Cyclodipeptide synthases (CDPSs) use aminoacylated tRNA (aa-tRNA) substrates to form peptide bonds between two amino acids yielding a cyclic dipeptide product (CDP). ParaCDPS from Parabacteroides sp. 20_3 (GenBank: EFK64745.1) produces cyclo(His-Phe)8 whilst ParcuCDPS from Parcubacteria bacterium RAAC4_OD1_1 (GenBank: ETB63777.1) can synthesise both cyclo(His-Glu) and cyclo(His-Pro)9. ParcuCDPS belongs to the XYP sub-group of the CDPS family, characterised by the presence of 3 residues: X40 where X is a non-conserved residue, Y202, and P203 (numbering respective to AlbC). ParcuCDPS displays a Rossman-fold common throughout the CDPS family.

Inspired by HisRS and histidine recognition more generally, and by the only high resolution structure of a CDPS with a ligand bound, we systematically altered three unique residues in ParcuCDPS P1, which we hypothesised to be participating in crucial interactions with the polar side chain of histidine. We first designed Generation 1 containing seven P1 mutants (Y55F; Y55V; E174A; E174H; E174L; Y189F and Y189L), and these variants were cloned, expressed in E.coli, purified and used for activity assays. By mutating the P1 residues, the activity of the variants was vastly reduced with E174A and E174H incapable of tolerating histidine as a substrate. Further investigation into the changes imposed by these mutants was performed by solving the crystal structures of a select few mutants containing changes to the active site or the pocket residues. The mutant structures were able to be solved using WT as a model and retained an equivalent fold to ParcuCDPS (Supplementary Notes 4 and 7 relating to Supplementary Figs. 13 and 14). Therefore, the disruption of activity is caused exclusively by the change in these few residues which appear important for the enzyme to produce a CDP. Having hindered the capacity of ParcuCDPS to recognize histidine, we then focussed on Generation 3 composed of three double mutants (Y55V + E174L; Y55V + Y189L; E174L + Y189L) and a triple mutant (Y55V + E174L + Y189L), aimed at switching the substrate specificity to a less polar amino acid. This was because Generation 1 and 2 variants essentially incorporate hydrophobic and non-polar amino acids potentially altering the overall environment and electrostatics of P1.

> MELHQIRGCHKNDIELKKYNIGVAISLGNKWFSIDNIEKLVKWSLLHTKEYVIIYIADSIHGINLSVRNKLSDSHAEEVAIRYGRNLFIKIKERVSLSFSQDEQAKIIYATWSDIADSKYKEKVKYLYNLYDKNINFKNYIENFVKEWVSKEKRTFNNNEINKFGRYILEELPLLMVQVKARGVLFEAYVYPYKTRITEFVGLLQKGEIFPEIKTNILDNHPKIFLEVRE>MGVVEEAHNVKVIGSGEATIVLGHGFGTDQSVWKHLVPHLVDDYRVVLYDNMGAGTTNPDYFDFDRYSNLEG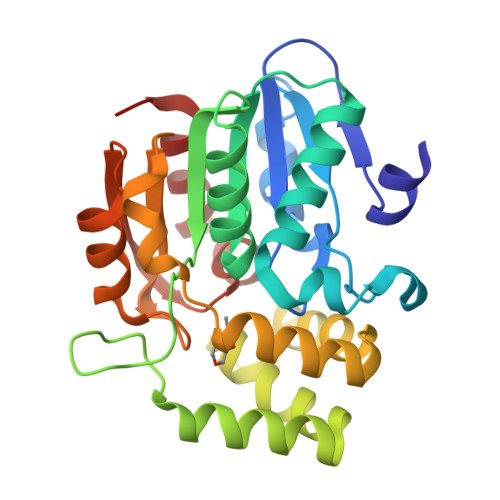YSFDLIAILEDLKIESCIFVGHSVSAMIGVLASLNRPDLFSKIVMISASPRYVNDVDYQGGFEQEDLNQLFEAIRSNYKAWCLGFAPLAVGGDMDSIAVQEFSRTLFNMRPDIALSVGQTIFQSDMRQILPFVTVPCHILQSVKDLAVPVVVSEYLHANLGCESVVEVIPSDGHLPQLSSPDSVIPVILRHIRNDIAM[2x]>[6x]MTRLTPDVLRMRSSQLSLRSLAMEQPQQRTAAPPTIDEAPTVPLEAKDLRPEHFTQPYLDFMTHNPTVFHVVDYCKQKLLKAGYVELPARDSWTGKLVPGGKYFTTRNGSSIIAFTVGQAYKPGNGIAMIAGHIDALTARLKPTSVKPTKEGYVQLGVAQYAGALNETWWDRDLSVGGRVIVKDPKTGKTTVKLVKVDWPVARIPTLAPHFGIGMTGHGNRETEMVPVIGIDNSDLLGEKAESEKPVGKPGSFASTQPPKLVKLILSQLGLSDPDSILNWELELFDAQPATVGGLDKEFIFAGRIDDKLCSWAAFMALLHAKRAPTDGVIKLVALFDDEEIGSLLRQGARGNFLPITIERILESFCSSNSVPFGPGILGQTYARSFLVSSDVTHAAHPNFTQT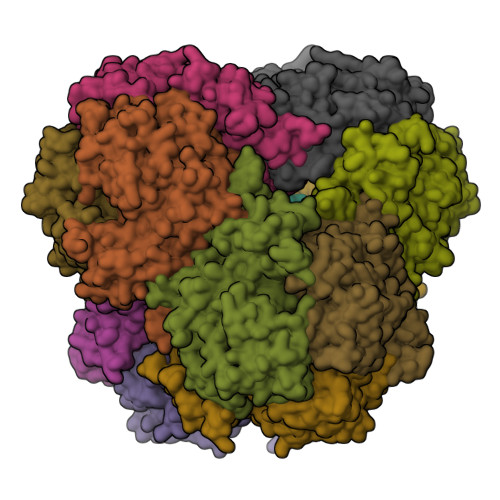NLPGHSPRLNVGVALCVDASAHMTTDSVSMAILDRIAELSGCVNQRHMIRNDSRSGGTVGPMLSAAMGVKAADVGIPQLSMHSIRAMTGSLDPGLGVKFYKGFLDFWEEVDLEWSH> MELIGDYSKAFLLQTVDGKHQDLKYISPETMV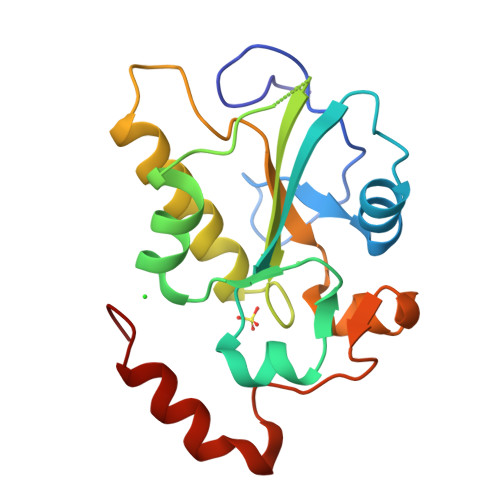ALLTGKFSNIVDKFVIVDCRYPYEYEGGHIKTAVNLPLERDAESFLLKSPIAPCSLDKRVILIFHSEFSSERGPRMCRFIRERDRAVNDYPSLYYPEMYILKGGYKEFFPQHPNFCEPQDYRPMNHEAFKDELKTFRLKTRSW(2S,3R,4E)-2-(hexadecanoylamino)-3-hydroxyoctadec-4-en-1-yl dihydrogen phosphate | C34 H68 N O6 P 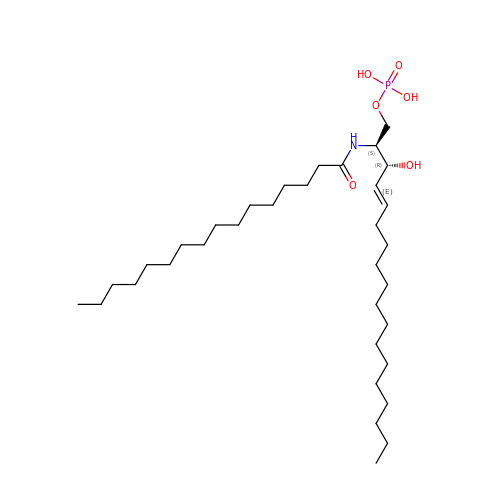| UNRULDRRONAKLU-TURZORIXSA-N>ATAAEIAALPRQKVELVDPPFVHAHSQVAEGGPKVVEFTMVIEEKKIVIDDAGTEVHAMAFNGTVPGPLMVVHQDDYLELTLINPETNTLMHNIDFHAATGALGGGGLTEINPGEKTILRFKATKPGVFVYHCAPPGMVP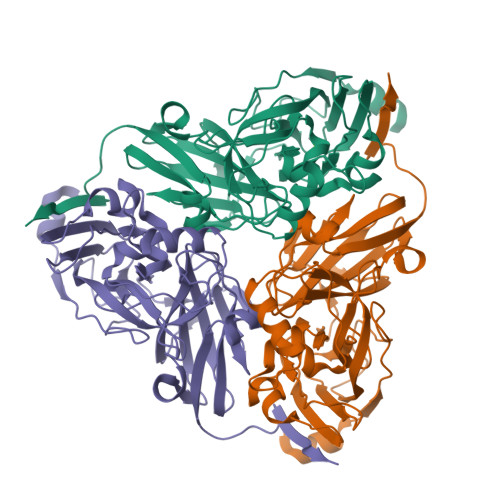WHVVSGGNGAIMVLPREGLHDGKGKALTYDKIYYVGEQDFYVPRDENGKYKKYEAPGDAYEDTVKVMRTLTPTHVVFNGAVGALTGDKAMTAAVGEKVLIVHSQANRDTRPHLIGGHGDYVWATGKFNTPPDVDQETWFIPGGAAGAAFYTFQQPGIYAYVNHNLIEAFELGAAAHFKVTGEWNDDLMTSVLAPSG[3x]>[4x]GIDPFTMSDLPCPPTNAERLHEFHRAIGAATPERPTPPPPELLRLRQTLLDEESAEVRAEIDHLLARQAAGEALSAGDLAPLAHELADLLYVTYGALDQLGIDADAVFAEVHR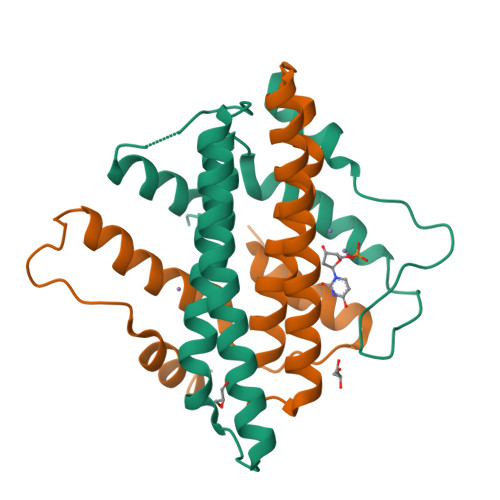ANLSKASGPRRADGKQLKPEGWRPADVRGVIERLQHAPADD> MLKKNDIVEVEIVDLTHEGAGVAKVDGLVFFVENALPSEKILMRVLKVNKKIGFGKVEKYLVQSPHRNQDLDLAYLRSGIADLGHLSYPEQLKFKTKQVKDSLYKIAGIADVEVAETLGMEHPVKYRNKAQVPVRRVNGVLETGFFRKNSHNLMPLEDFFIQDPVIDQVVVALRDLLRRFDLKPYDEKEQSGLIRNLVVRRGHYSGQIMVVLVTTRPKVFRVDQLIEQVIKQFPEIVSVMQNI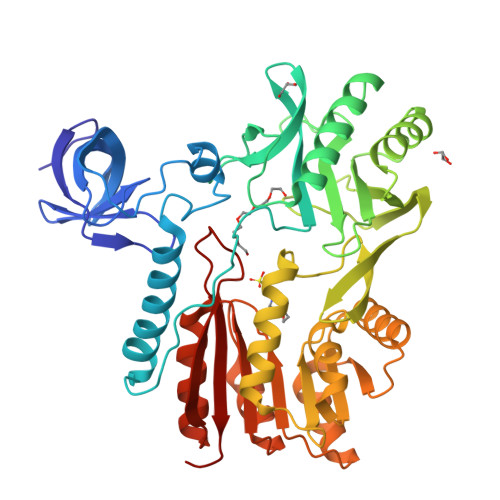NDQNTNAIFGKEWRTLYGQDYITDQMLGNDFQIAGPAFYQVNTEMAEKLYQTAIDFAELKKDDVIIDAYSGIGTIGLSVAKHVKEVYGVELIPEAVENSQKNASLNKITNAHYVCDTAENAMKKWLKEGIQPTVILVDPPRKGLTESFIKASAQTGADRIAYISCNVATMARDIKLYQELGYELKKVQPVDLFPQTHHVETVALLSKLDVD>GHMNKMNIDKNLLEKWDKEYIWHPYTQMKEYRESKNLIIERGEGNYLIDIYGNKYLDAVSSIWCNLFGHSRKEIIEAIKNQADKICHSTLLGCGNVPSILLAKKLVDITPKHLTKVFYSEDGAEAVEIAIKMAYQYYVLRGDKGRTKFISVKEGYHGDTVGAMSVGGSELFHGVFKPLLFKGYHANPPYCYRCKYHNFKDTDERNEKGCEMECLNEMISLIEKHAEEVFCVILEGGIMGSAGMIPYPDGYIEGVAKACKENDVIFILDEVATGFGRTGKMFFCDNEELKKLEKPDILCLGKGLTGGYLPLAATLTTDEIYNQFLGEFGESKQLYHGHTYTGNQLLCSAALATLEIFEKENVIE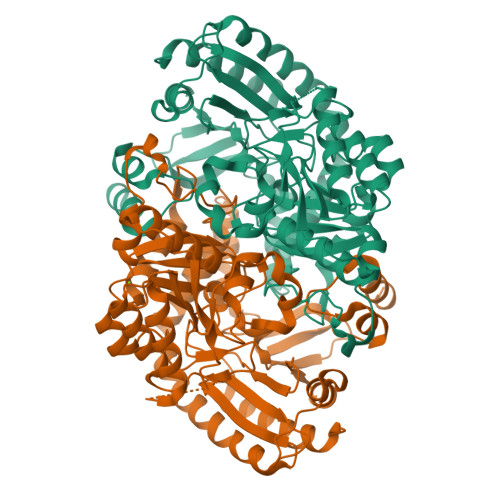NIQPKIKLFHKELRKLKELEHVGDVRGRGFMVGIELVKDKETKEPYPYGYKAGYRVAEKLLEKGIYMRPIGNVIILVPPLSITEKEIIYLCDALYEAIKEADL[2x]> MSTSLLFEQLNFLILVAAEAELPIAHSTRKLLMDNSCNNCQIYELYNENLKDVKTDKDWFMNKFGPQTVHFVISNTINFPFYKIVYFDLLIPVVSHTWVQDSVKTKRHLRTNMYSPNPFHLLRDCQVYISKSSFNKCEYILYSDLLHLLGGTLVNYISNRTTHVIVQSPQDPIIATVSKLTFGSFSSSSTNKHTEKPLREWKFVYPIWILYHFKMAKPLKGELATLCEL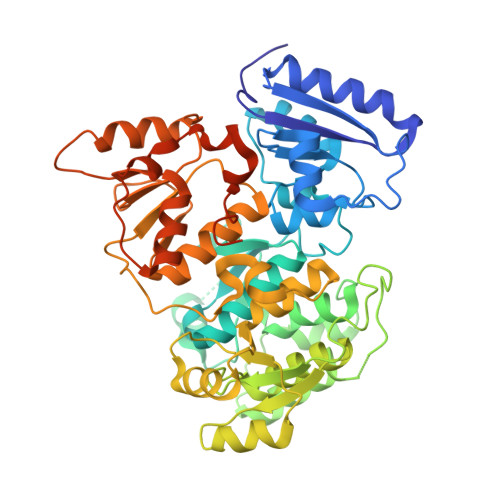DMQDTSEEQLFAKWEEVIGDKQTSSSQLTLHPNKTLFKNHHFAISPDLNFFTPLYWFLKGFIEDLDGKVTPLSFSDDLKSVYQAFPDIDCYIGHSANSPILEKTKSIKPEIHVGNVSWLFYMFALQKFTPVSQCKLIHQPFHAKLFTSKELTVAYTNYFGSQRFYIQRLVEILGGLSTPELTRKNTHLITKSTIGKKFKVAKKWSLDPQNAIIVTNHMWLEQCYMNNSKLNPKDSRFQNFKLDDNMGWNIGQIGMDHSSLPTPKNLSMVTYDTQSISEKPPPTN> MAEQINENYENKQQLVEQTEITTFENDLIVLEDGPQMEESLPFAFHGQHTDNRQHTVVNFLQRPQVIFDSSWASDVPRNKQFMDSIMIPDDIISFPMFAEKLKGFSSLRATAVITVQFQTQPFQAGRVMLGSFPLPTLNPTRVKFATNHVSRLMLLNHVQCDIAKETEVSLRIPFVSPYNSY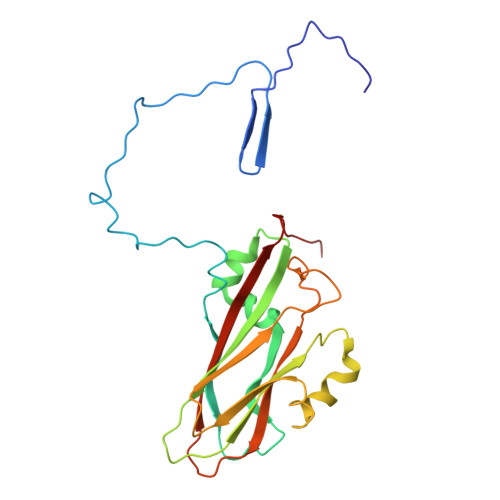DLVSKRFPWAKVVGLVYSPLTTTIPVDFIVYGHFEDVELGCPTSGMLAQ>[2x]SSWAAELAKPLTLDQLQQQNGKAIDTRPSAFYNGWPQTLNGPSGHELAALNLSASWLDKMSTEQLNAWIKQHNLKTDAPVALYGNDKDVDAVKTRLQKAGLTHISILSDALSEPSRLQKLPHFEQLVYPQWLHDLQQGKEVTAKPAGDWKVIEAA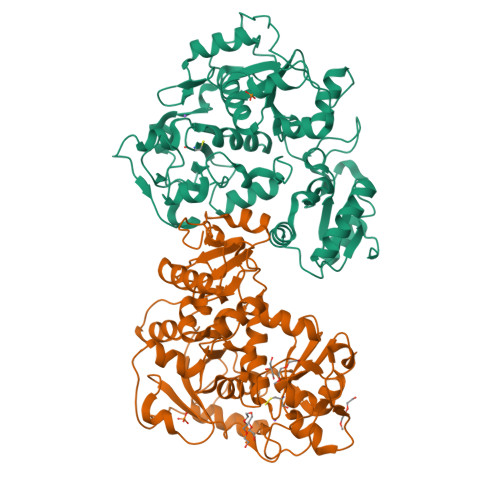WGAPKLYLISHIPGADYIDTNEVESEPLWNKVSDEQLKAMLAKHGIRHDTTVILYGRDVYAAARVAQIMLYAGVKDVRLLDGGWQTWSDAGLPVERGTPPKVKAEPDFGVKIPAQPQLMLDMEQARGLLHRQDASLVSIRSWPEFIGTTSGYSYIKPKGEIAGARWGHAGSDSTHMEDFHNPDGTMRSADDITAMWKAWNIKPEQQVSFYCGTGWRASETFMYARAMGWKNVSVYDGGWYEWSSDPKNPVATGERGPDSSK>MKYVVVSGGVISGIGKGVLASSTGMLLKTLGLKVTSIKIDPYMNIDAGTMSPLEHGECFVLDDGGETDLDLGNYERYLGITLSRDHNITTGKIYSHVISRERRGDYLGKTVQIVPHLTNAIQDWIQRVSKIPVDDTGLEPDVCIIELGGTVGDIESAPFVEALRQFQFEVGRENFALIHVSLVPVIHGEQKTKPTQAAIKDLRSLGLIPDMIACRCSEELNRSTIDKIAMFCHVGPEQVVNVHDVNSTYHVPLLLLKQHMIDYLHSRLKLGEVPLTLEDKERGSQLLTNWENMTKNLDDSDDVVKIALVGKYTNLKDSYLSVTKSLEHASMKCRRQLEILWVEASNLEPETQEVDKNKFHDSWNKLSSADGILVPGGFGTRGIEGMILAAKWARESGVPFLGVCLGLQVAAIEFARNVIGRPNSSSTEFLDETLLAPEDQVVITMRLGLRPTIFQPNSEWSNIRKLYGEVNEVHERHRHRYEINPKIVNDMESRGFIFVGKDETGQRCEIFELKGHPYYVGTQYHPEYTSKVLEPSRPFWGLVAAASGTLGEVIKDINL[16x]

CTP synthase (CTPS) catalyzes the final, rate-limiting step of de novo CTP biosynthesis (Lieberman, 1956). Each CTPS monomer consists of a glutaminase domain and an amido-ligase domain connected by an alpha helical linker. Glutamine hydrolysis in the glutaminase domain produces ammonia which is transferred through a channel into the amido-ligase domain, where it is ligated to UTP to form CTP in an ATP-dependent process. Budding yeast have two CTPS isoforms, Ura7 and Ura8, which share 78 % identical residues.

We determined structures of CTPS filament bundles formed at pH 6.0 to better understand the mechanisms of lateral assembly. As we found for the single filament structures, Ura8 reconstructions went to higher resolution (3.3 Å for substrates and 3.7 Å for product) than Ura7 (6.6 Å substrate and 7.0 Å product). The Ura8 substrate-bound structure had the same architecture as both Ura7 bundles, but the product-bound Ura8 structure had very different interfaces between filaments, giving rise to filaments in register. To better understand the nature of lateral assembly contacts, we built atomic models into the two Ura8 bundle structures. Ligands were clearly visible, and bound as in the single filament structures, and the longitudinal assembly interfaces were the same as observed in the single filaments. Yeast CTPS has a 7-residue insert (residues 273–279) in the linker region that mediates the bulk of the lateral interaction in both bundle types. In the product-bound structure the linker inserts near the tetramerization interface and packs against Pro236 and Ile225. The buried surface area per tetramer at lateral interfaces, 2202 Å2 (substrates-bound) or 1676 Å2 (product-bound), is comparable to the 2460 Å2 involved in longitudinal filament assembly contacts, suggesting that lateral association contributes to the overall stability of the assembly. Propagation of trans interactions in the Ura8 product bound structure with filaments in register also results in a curved sheet, but propagation of cis interactions results in a closed tube with nine filaments. Conversely, Ura8 forms bundles with radically different architectures dependent on whether substrates or products are bound; it remains unclear what the functional consequence is of having two distinct bundle architectures.> SAECPVVNELERINCIPDQPPTKATCDQRGCCWNPQGAVSVPWCYYSKNHSYHVEGNLVNTNAGFTARLKNLPSSPVFGSNVDNVLLTAEYQTSNRFHFKLTDQTNNRFEVPHEHVQSFSGNAAASLTYQVEISRQPFSIKVTRRSNNRVLFDSSIGPLLFADQFLQLSTRLPSTNVYGLGEHVHQQYRHDMNWKTWPIFNRDTTPNGNGTNLYGAQTFFLCLEDASGLSFGVFLMNSNAMEVVLQPAPAITYRTIGGILDFYVFLGNTPEQVVQEYLELIGRPALPSYWALGFHLSRYEYGTLDNMREVVERNRAAQLPYDVQHADIDYMDERRDFTYDSVDFKGFPEFVNELHNNGQKLVIIVDPAISNNSSSSKPYGPYDRGSDMKIWVNSSDGVTPLIGEVWPGQTVFPDYTNPNCAVWWTKEFELFHNQVEFDGIWIDMNEVSNFVDGSVSGCSTNNLNNPPFTPRILDGYLFCKTLCMDAVQHWGKQYDIHNLYGYSMAVATAEAAKTVFPNKRSFILTRSTFAGSGKFAAHWLGDNTATWDDLRWSIPGVLEFNLFGIPMVGPDICGFALDTPEELCRRWMQLGAFYPFSRNHNGQGYKDQDPASFGADSLLLNSSRHYLNIRYTLLPYLYTLF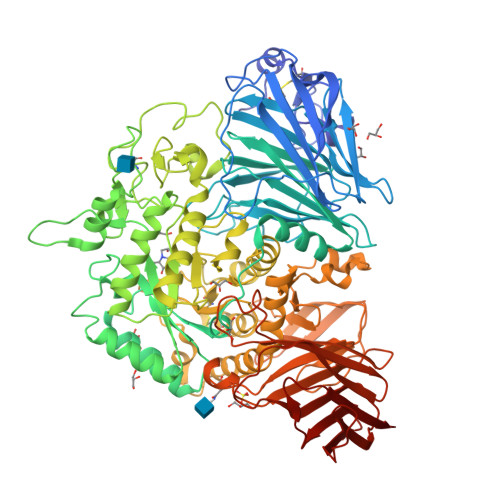FRAHSRGDTVARPLLHEFYEDNSTWDVHQQFLWGPGLLITPVLDEGAEKVMAYVPDAVWYDYETGSQVRWRKQKVEMELPGDKIGLHLRGGYIFPTQQPNTTTLASRKNPLGLIIALDENKEAKGELFWDDGETKDTVANKVYLLCEFSVTQNRLEVNISQSTYKDPNNLAFNEIKILGTEEPSNVTVKHNGVPSQTSPTVTYDSNLKVAIITDIDLLLGEAYTVEWAH> GPVEDAITAAIGRVADTVGTGPTNSEAIPALTAAETGHTSQVVPGDTMQTRHVKNYHSRSESTIENFLCRSACVYFTEYKNSGAKRYAEWVLTPRQAAQLRRKLEFFTYVRFDLELTFVITSTQQPSTTQNQDAQILTHQIMYVPPGGPVPDKVDSYVWQTSTNPSVFWTEGNAPPRMSIPFLSIGNAYSNFYDGWSEFSRNGVYGINTLNNMGTLYARHVNAGSTGPIKSTIRIYFKPKHVKAWIPRPPRLCQYEKAKNVNFQPSGVTTTRQSITTMTNTGAF;> SPTVEECGYSDRARSITLGNSTITTQECANVVVGYGVWPDYLKDSEATAEDQPTQPDVATCRFYTLDSVQWQKTSPGWWWKLPDALSNLGLFGQNMQYHYLGRTGYTVHVQCNASKFHQGCLLVVCVPEAEMGCATLDNTPSSAELLGGDTAKEFADKPVASGSNKLVQRVVYNAGMGVGVGNLTIFPHQWINLRTNNSATIVMPYTNSVPMDNMFRHNNVTLMVIPFVPLDYCPGSTTYVPITVTIAPMCAEYNGLRLAGHQ;> GLPTMNTPGSCQFLTSDDFQSPSAMPQYDVTPEMRIPGEVKNLMEIAEVDSVVPVQNVGEKVNSMEAYQIPVRSNEGSGTQVFGFPLQPGYSSVFSRTLLGEILNYYTHWSGSIKLTFMFCGSAMATGKFLLAYSPPGAGAPTKRVDAMLGTHVIWDVGLQSSCVLCIPWISQTHYRFVASDEYTAGGFITCWYQTNIVVPADAQSSCYIMCFVSACNDFSVRLLKDTPFISQQNFFQ;> MGAQVSTQKTGAHETRLNASGNSIIH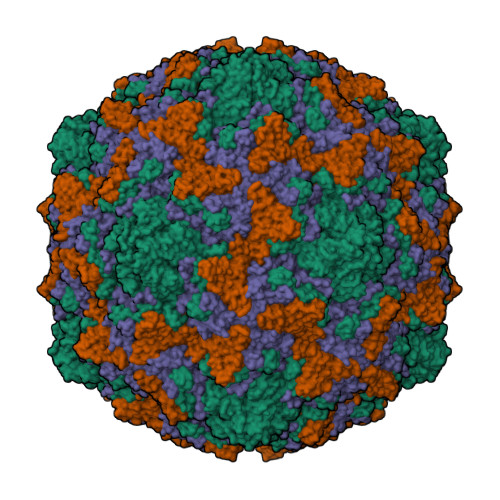YTNINYYKDAASNSANRQDFTQDPGKFTEPVKDIMIKSLPALN>[4x]MRGSHHHHHHGMASMELSSLTAVSPVDGRYGDKVSALRGIFSEYGLLKFRVQVEVRWLQKLAAHAAIKEVPAFAADANGYLDTLVANFNEEDAARIKTIERTTNHDVKAVEYFLKEKVAAIPALHDVSEFIHFACTSEDINNLSHALMLKTARDEVILPYWRQVINAVKDLATQYRDIPLLSRTHGQPATPSTLGKEMANVAYRMERQ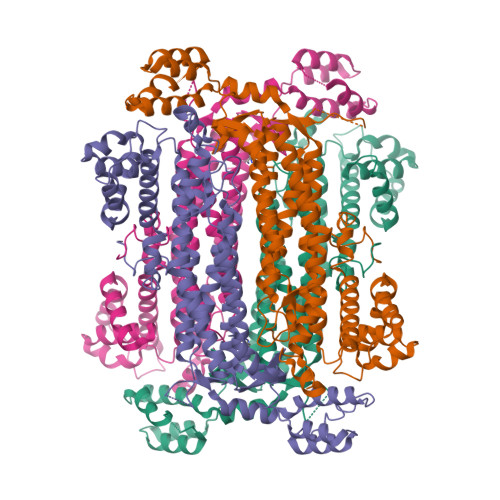FRQLNQVEILGKINGAVGNYNAHIAAYPEVDWHQFSEEFVTSLGIQWNPYTTQIEPHDYIAELFDCIARFNTILIDFDRDVWGYIALNHFKQKTIAGEIGSSTMPHKVNPIDFENSEGNLGLSNAVLHHLANKLPVSRWQRDLTDSTVLRNLGVGIGYALIAYQSTLKGVSKLEVNRDHLLDELDHNWEVLAEPIQTVMRRYGIEKPYEKLKELTRGKRVDAEGMKQFIDSLALPEAEKTRLKAMTPANYIGRAVTLVDELK> GQSVPWGISRVQAPAAHNRGLTGSGVKVAVLDTGISTHPDLNIRGGASFVPGEPSTQDGNGHGTHVAGTIAALNNSIGVLGVAPSAELYAVKVLGADGRGAISSIAQGLEWAGNNGMHVANLSLGSPSPSATLEQAVNSATSRGVLVVAASGNSGASSISYPARYANAMAVGATDQNNNRASFSQYGAGLD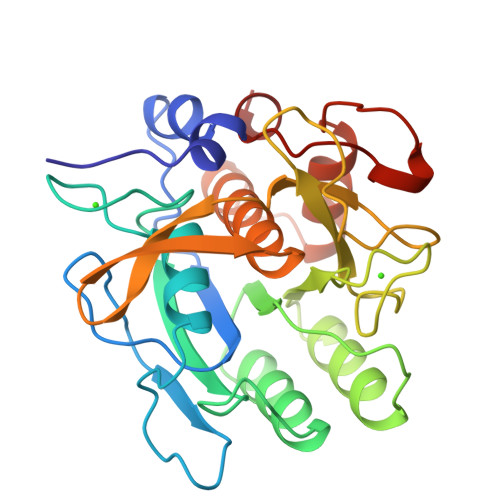IVAPGVNVQSTYPGSTYASLNGTSMATPHVAGAAALVKQKNPSWSNVQIRNHLKNTATSLGSTNLYGSGLVNAEAATR> MGSVQRQDLVLFSDQSVLPAHFFQDSNSH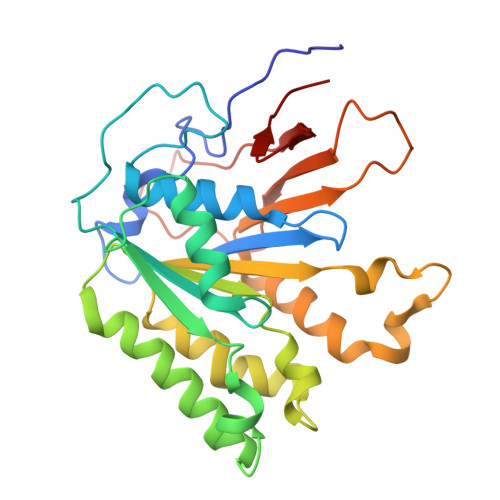NLFFITHQSCTQPLWMINALVETHVLGSPSSLNESSSSMLPSSTRSHAVLASFIHEQNYFTNSLNKLKIPSNNYNVLDFLSDFIVNNIHNKPRDKILSDVLAKFSAAIQNNPTDTIVIIEQPELLLSLVSGLTCSELNNKFITPLLRQCKVLIIVSNSDIFNIDEYDASVHSSNLQNFYKSSFIKSMINLNLNPLKTGFAKDVTGSLHVCRGGAPIATSNTSLHVVENEYLYLNEKESTKLFYR>[12x]ERPTLKTIAYMTGLGITTVSRALKDAPDIGAETKERVRLI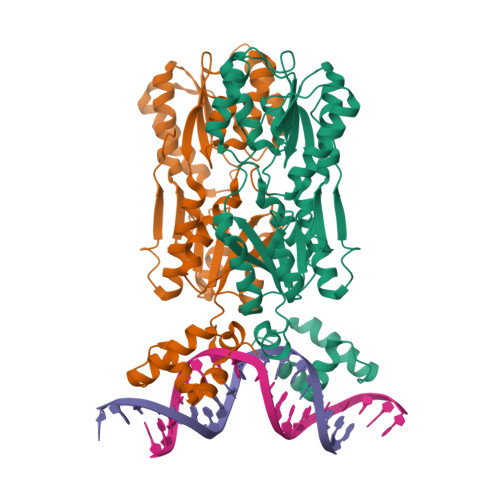AQQIGYQPNRAGVRLRTGKTNVIALVLSVDEELMGFTSQMVFGITEVLATTQYHLVVTPHTHAKDSMVPIRYILETGSADGVIISKIEPNDPRVRFMTERKMPFVTHGRSDMGIEHAYHDFDNEAYAYEAVERLAQCGRKRIAIIVPPSRFAFHDHARKGFTRGIRDFGVSEFPLDAITIETPLDKIRDFGKRLMQSDDRPDGIVSISGSSTIALVAGFEAAGVRIGKDIDIVSKQSAEFLNWIQPQIHTVNEDIKLAGRELAKALLARINGAPPETLQSVSRPVWSSMAPKPLEHHHHHH> MRLLKYPL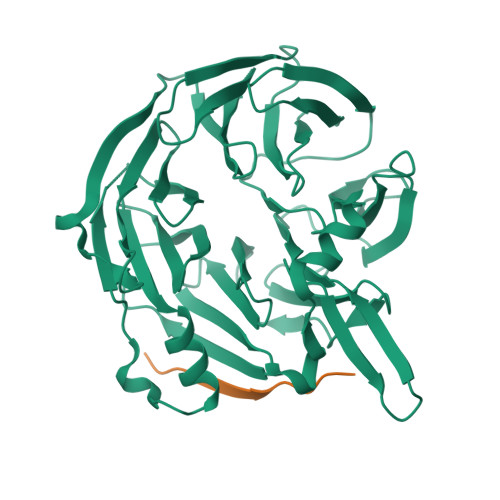DIHNEQVNALAALGPYIILAGSGGHVMAWRQQQLVDTAFDRVMIKDLKPEVSFQVDQDTTGDIFFITGDLETLYIGSEHRLWGYSGWLCRDTNNINSVEKMNSKLLFECKSPSTITDVKYDINLGILFVLLSNENKILLFRHKTFDKLSEITIDKASKPITGIIDPTGQTFTVMTSDRSILVYQINKTGTHKLINKLTQHVQMYPLHYRISMSPQADILPVINSVKGVPNNATSCTALLDRNNNYKVTKTLVTPSSNGCRVLVYSPAFYEKPNLKKGTSTRYNLIATSGSTDGTILVWNTKRMKPLFNALQVSSTAINDMSWSQDGFTLFAISNDATLYTFAFQEKDLGVALPQTEIKSLQEVNK;> KEPSILIDVPLYQADTNDYLD(1~{R},3~{R})-5-[(2~{E})-2-[(1~{R},3~{a}~{S},7~{a}~{R})-1-[(2~{R},6~{R})-6-(4-hydroxyphenyl)-6-methoxy-hexan-2-yl]-7~{a}-methyl-2,3,3~{a},5,6,7-hexahydro-1~{H}-inden-4-ylidene]ethylidene]-2-methylidene-cyclohexane-1,3-diol 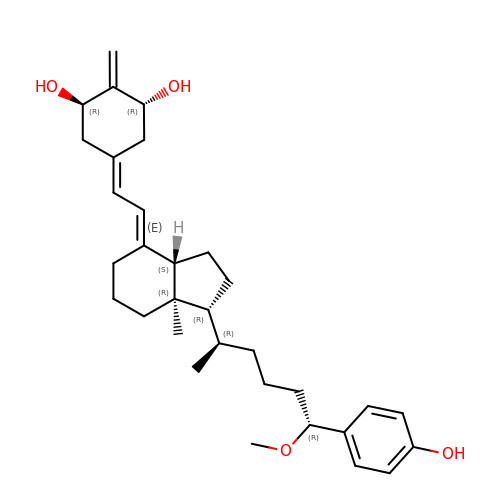| C32 H46 O4 | LNLTYAYGVNOEBQ-OJABYWBNSA-N>VEHPEFLKAGKEPGLQIWRVEKFDLVPVPPNLYGDFFTGDAYVILKTVQLRNGILQYDLHYWLGNECSQDESGAAAIFTVQLDDYLNGRAVQHREVQGFESATFLGYFKSGLKYKKGGVASGFKHVVPNEVVVQRLLQVKGRRVVRATEVPVSWESFNNGDCFILDLGNNIYQWCGSKSNRFERLKATQVSKGIRDNERSGRAQVSVFEEGAEPEAMLQVLGPKPTLPEATEDTVKEDAANRKLAKLYKVSNGAGPMVVSLVADENPFAQGALRSEDCFILDHGKDGKIFVWKGKQANMEERKAALKTASDFISKMDYPKQTQVSVLPEGGETPLFRQFFKNWRDPDQTEGLGLAYLSSHIAHVERVPFDAATLHTSTAMAAQHGMDDDGTGQKQIWRVEGSNKVPVDPATYGQFYGGDSYIILYNYRHGSRQGQIIYNWQGAQSTQDEVAASAILTAQLDEELGGTPVQSRVVQGKEPAHLMSLFGGKPMIVYKGGTSREGGQTAPASTRLFQVRASSSGATRAVEIIPKAGALNSNDAF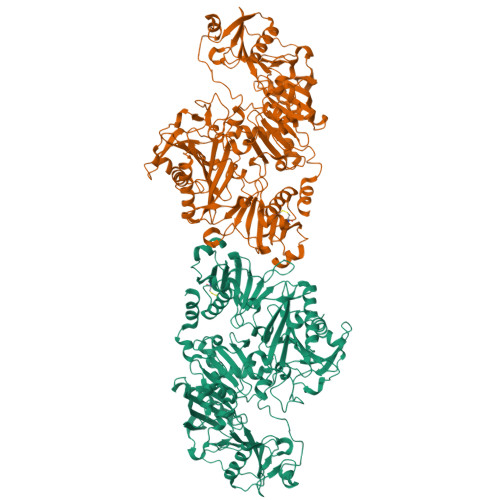VLKTPSAAYLWVGAGASEAEKTGAQELLRVLRAQPVQVAEGSEPDSFWEALGGKATYRTSPRLKDKKMDAHPPRLFACSNKIGRFVIEEVPGEFMQEDLATDDVMLLDTWDQVFVWVGKDSQDEEKTEALTSAKRYIDTDPAHRDRRTPITVVKQGFEPPSFVGWFLGWDDSYWSVDPLDRALAELAA[2x]>[4x]MMVIDTSALVAMLSDEPDAERFEAAVEADHIRLMSTASYLETALVIEARFGEPGGRELDLWLHRAAVDLVAVHADQADAARAAYRTYGKGRHR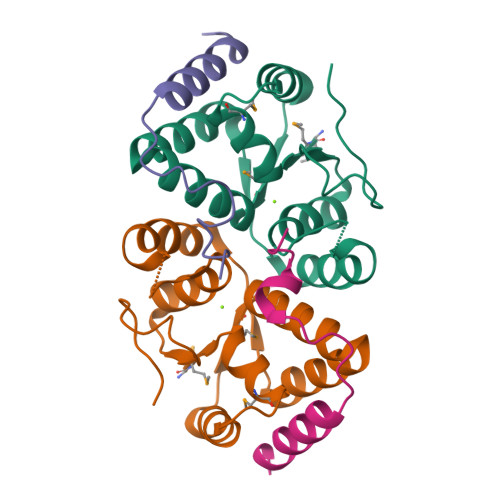AGLNYGDCFSYGLAKISGQPLLFKGEDFQHTDIATVALP;>[4x]MALSIKHPEADRLARALAARTGETLTEAVVTALRERLARETGRARVVPLRDELAAIRHRCAALPVVDNRSAEAILGYDERGLPA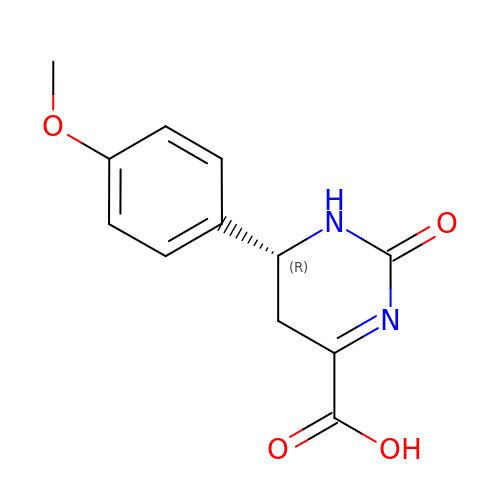(6~{R})-6-(4-methoxyphenyl)-2-oxidanylidene-5,6-dihydro-1~{H}-pyrimidine-4-carboxylic acid | C12 H12 N2 O4 | MTFBEIOPWWFNND-SECBINFHSA-N4-(4-HYDROXY-3-ISOPROPYLPHENYLTHIO)-2-ISOPROPYLPHENOL | C18 H22 O2 S 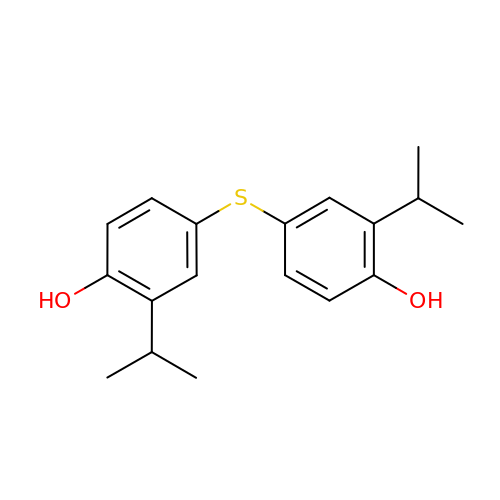| NEMLLZAROZVCCE-UHFFFAOYSA-N>ATVPLPAEGEIGLVHIGALTLENGTVLPDVTIAVQRWGELAPDRGNVVMVLHALTGDSHVTGPAGDGHPTAGWWDGVAGPGAPIDTDHWCAIATNVLGGCRGSTGPGSLAPDGKPWGSRFPQITIRDQVAADRAALAALGITEVAAVVGGSMGGARALEWLVTHPDDVRAGLVLAVGARATADQIGTQSTQVAAIKADPDWQGGDYHGTGRAPTEGMEIARRFAHLTYRGEEELDDRFANTPQDDEDPLTGGRYAVQSYLEYQGGK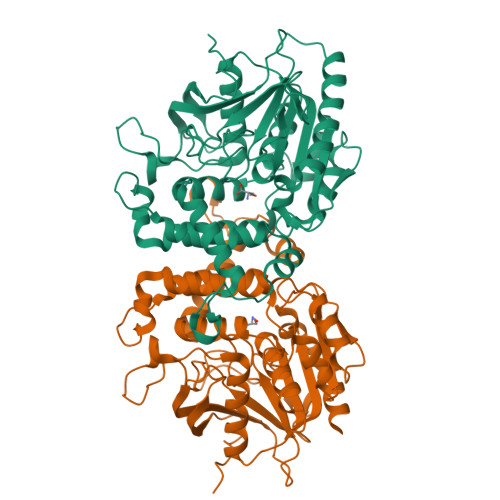LARRFDPGTYVVLSDALSSHDVGRGRGGVEAALRSCPVPVVVGGITSDRLYPIRLQQELAELLPGCQGLDVVDSIYGHDGFLVETELVGKLIRRTLELAQRLEHHHHHH[2x]>[4x]XGELAAIKQ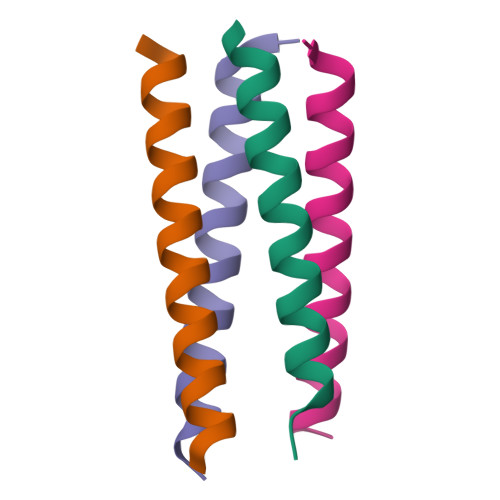ELAAIKKELAAIKWELAAIKQGAGX>[2x]MDSQRNLLVIALLFVSFMIWQAWEQDKNPQPQAQQTTQTTTTAAGSAADQGVPASGQGKLISVKTDVLDLTINTRGGDVEQALLPAYPKELNSTQPFQLLETSPQFIYQAQSGLTGRDGPDNPANGPRPLYNVEKDAYVLAEGQNELQVPMTYTDAAGNTFTKTFVLKRGDYAVNVNYNVQNAGEKPLEISTFGQLKQSITLPPHLDTGSSNFALHTFRGAAYSTPDEKYEKYKFDTIADNENLNISSKGGWVAMLQQYFATAWIPHNDGTNNFYTANLGNGIAAIGYKSQPVLVQPGQTGAMNSTLWVGPEIQDKMAAVAPHLDLTVDYGWLWFISQPLFKLLKWIHSFVGNWGFSIIIITFIVRGIMYPLTKAQYTSMAKMR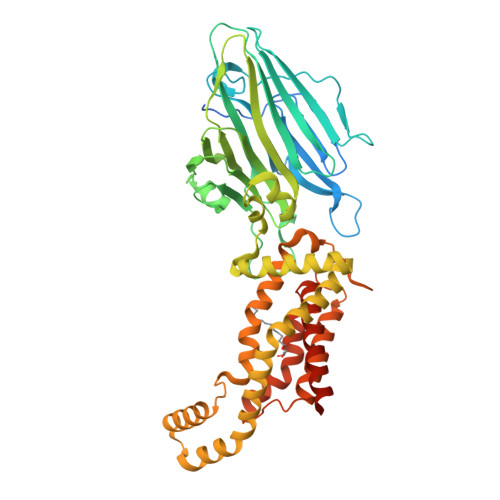MLQPKIQAMRERLGDDKQRISQEMMALYKAEKVNPLGGCFPLLIQMPIFLALYYMLMGSVELRQAPFALWIHDLSAQDPYYILPILMGVTMFFIQKMSPTTVTDPMQQKIMTFMPVIFTVFFLWFPSGLVLYYIVSNLVTIIQQQLIYRGLEKRGLLESSGENLYFQ> KMART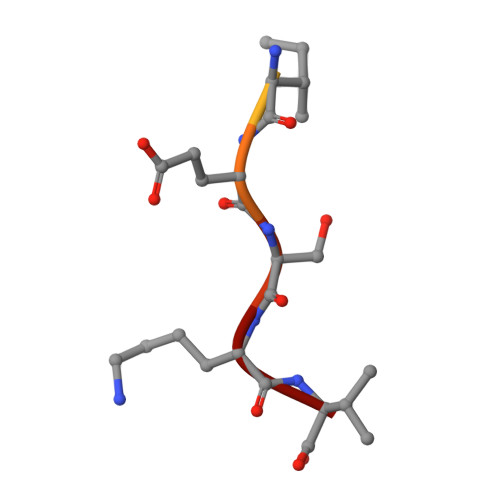IESKV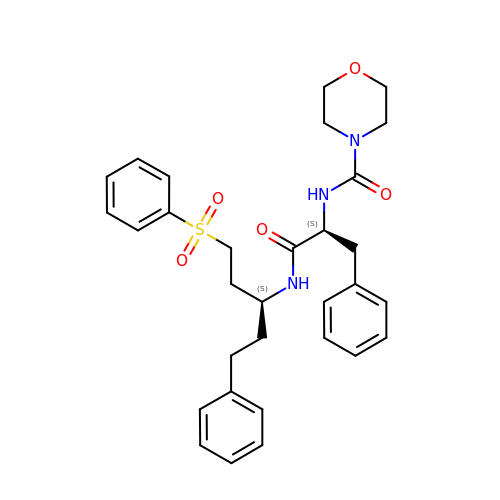3-[[N-[MORPHOLIN-N-YL]-CARBONYL]-PHENYLALANINYL-AMINO]-5- PHENYL-PENTANE-1-SULFONYLBENZENE | C31 H37 N3 O5 S | NNOXYPYTWAQTTO-YTMVLYRLSA-N> TSELRICRINKESGPCTGGEELYLLCDKVQKEDISVRFSTASWEGRGDFSQADVHRQIAIV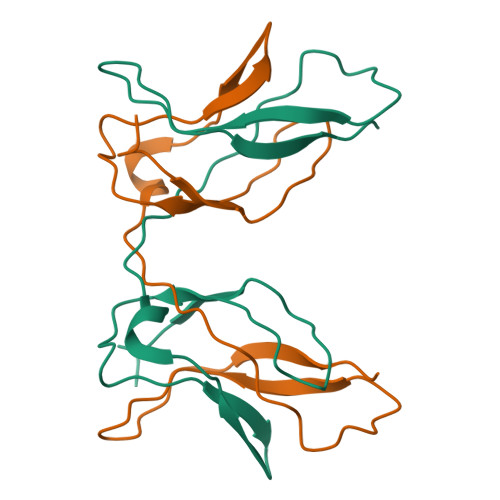FKTPPYEDLEISEPVTVNVQLQRLTDGECSEPLPFTYLPR{2-[(benzylsulfonyl)carbamoyl]-5-methoxy-1H-indol-1-yl}acetic 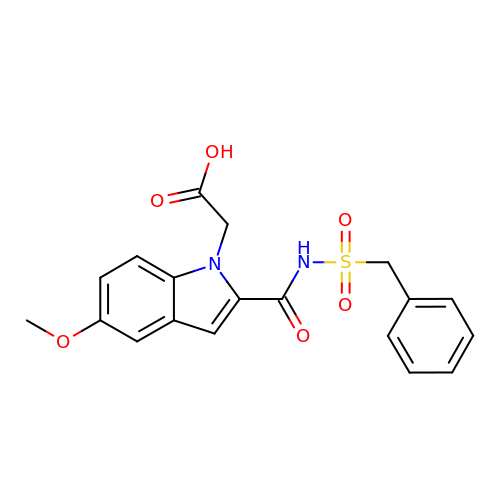acid | C19 H18 N2 O6 S | YVDIPFZVZYBIQS-UHFFFAOYSA-N> SVKGSVDL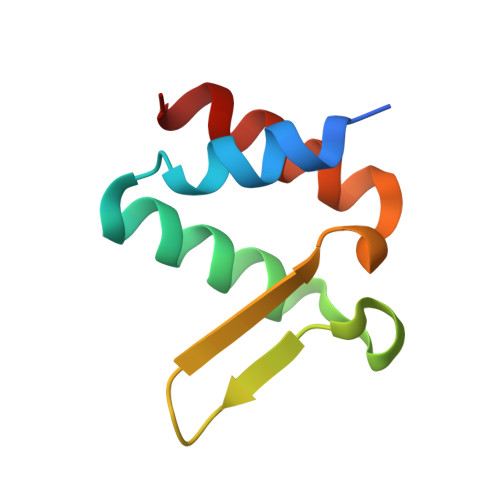EKLAFGLTKLNEDDLVGVVQMVTDNKTPEMNVTNNVEEGEFIIDLYSLPEGLLKSLWDYVKKNT>[2x]MGHHHHH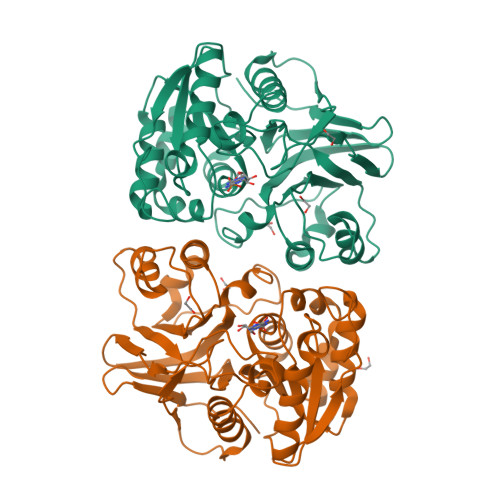HHHHHHHSSGHIDDDDKHMLEMIQSHPLLAAPLAVGDTIGFFSSSAPATVTAKNRFFRGVEFLQRKGFKLVSGKLTGKTDFYRSGTIKERAQEFNELVYNPDITCIMSTIGGDNSNSLLPFLDYDAIIANPKIIIGYSDTTALLAGIYAKTGLITFYGPALIPSFGEHPPLVDITYESFIKILTRKQSGIYTYTLPEKWSDESINFNENKILRPKKLYKNNCAFYGSGKVEGRVIGGNLNTLTGIWGSEWMPEIRNGDILFIEDSRKSIATVERLFSMLKLNRVFDKVSAIILGKHELFDCAGSKRRPYEVLTEVLDGKQIPVLDGFDCSHTHPMLTLPLGVKLAIDFDNKNISITEQYLSTEK>MTSTLQATDIATLSPNEQAAIDAWWRAANYLSVGQIYLRDNPLLQEPLRPEHIKQRLLGHWGSDPGLSFVYVHLNRLIRRLDLNLIYVTGPGHGAPALLANAWLEGTYSEVYPNCQQSTAGLQQFFKQFSFPGGIGSHCTPETPGSIHEGGELGYSLSHAFGAALDNPDLIVACVIGDGEAETGPLATSWHSNKFLNPAQDGAVLPILHLNGYKIANPTLLSRISHEELRSLFIGYGYEPFFVEGNDPAILHGVMASTLATCVQKIQAIQAAARSGESSDRPMWPMIVLRTPKGWTGPATIKGHVVEGSWRSHQVPMADVLTNPEHLQLLEDWLRSYRPEELFDASGAPVAELQAIAPIGDRRMSANPVTNGGLLRRALTLPDFRDQAVSVPAPGKSRADSTRPLGQFLREVIRHNPDNFRLFGPDETASNRLDAVYEVTSKVWLGDRIPEDEDGGHLSDRGRVMEILSEHTLEGWLEAYLLTGRHGFFATYEAFAHVIDSMVNQHAKWLDVSKREVDWRAPVSSLNILLSSTVWRQDHNGFSHQDPGFIDLVTNKSARVTRIYLPPDANCLLSVADHCLRSTDYINVIVADKQSHLQYLDAEAAARHCAKGIGIWDWASNDQGASPDVVIASCGDVVTLEALAATALLREHFPDLKIRFVNVVDLFRLQPDTEHPHGLSDRDFDSLFTVDKPIIFNFHGYPWLIHKLAYRRHNHNNLHVRGYKEVGNINTPLELAIRNQVDRFNLAIDVIDRVPHLRDRGAHVKEWLKDQIHDHIQYAYQEGIDRPEINQWQWPF[12x]

Phosphoketolase (XPK) belongs to the transketolase family, a member of thiamine pyrophosphate (TPP)-dependent enzyme superfamily. It converts F6P, xylulose-5-phosphate (Xu5P) or sedoheptulose-7-phosphate (S7P), which are intermediates in RuBP regeneration, to produce acetyl phosphate (AcP) and C3, C4 or C5 sugar phosphates. XPK is an enzyme present in many microorganisms, primarily involved in substrate-level phosphorylation to produce AcP.

Given the importance of the physiological role of SeXPK, we solved the cryo-EM structures of SeXPK, both free (with coenzyme TPP/Mg2+ bound) and complexed with the non-hydrolyzable ATP analog, AMPPNP. In contrast to the published XPK structures from Lactococcus lactis and B. breve/longum, which exist as dimers in crystals, the cryo-EM structure of SeXPK is a dodecamer composed of six dimeric units, forming a circular donut-shaped array both for the AMPPNP-bound form and in the absence of AMPPNP. Of note, while the dimer–dimer interface in the SeXPK dodecamer involves residues near the C terminus, the B. longum XPK octamer involves residues near the N terminus. As the donut-shape or four-leaf clover shape-like particles or two-dimensional (2D) class average images were not in perfect symmetry, we further examined whether the assigned symmetries were pseudosymmetry. Some relative random motions were observed between different dimers in both SeXPK dodecamer and B. longum octamer assemblies, suggesting the likelihood of pseudosymmetry in these structures. The root-mean-square deviation between the structures with and without AMPPNP-bound is very small: (0.42 Å from 7,897 Cα atoms of the dodecamer and 0.36 Å from 1,256 Cα atoms of the dimer).(4-{[(3R)-1-benzylpyrrolidin-3-yl]amino}-2-nitrophenyl)methanol 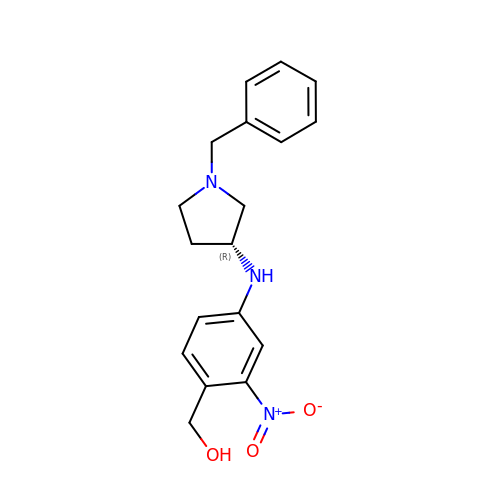| C18 H21 N3 O3 | BWQQLSMUSJPPCM-QGZVFWFLSA-N>MPHVENASETYIPGRLDGKVALVTGSGRGIGAAVAVHLGRLGAKVVVNYANSTKDAEKVVSEIKALGSDAIAIKADIRQVPEIVKLFDQAVAHFGHLDIAVSNSGVVSFGHLKDVTEEEFDRVFSLNTRGQFFVAREAYRHLTEGGRIVLTSSNTSKDFSVPKHSLYSGSKGAVDSFVRIFSKDCGDKKITVNAVAPGGTVTDMFHEVSHHYIPNGTSYTAEQRQQMAAHASPLHRNGWPQDVAN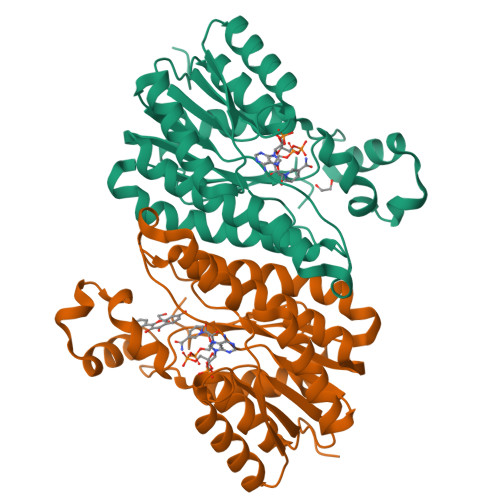VVGFLVSKEGEWVNGKVLTLDGGAA[4x]> PKQLRFEGERVTWIQASTLKELLDLKAQHPEAKLVVGNTEIGIEMKFKNQLFPMIICPAWIPELNAVEHGPEGISFGAACALSSVEKTLLEAVAKLPTQKTEVFRGVLEQLRWFAGKQVKSVASLGGNIITASPISDLNPVFMASGTKLTIV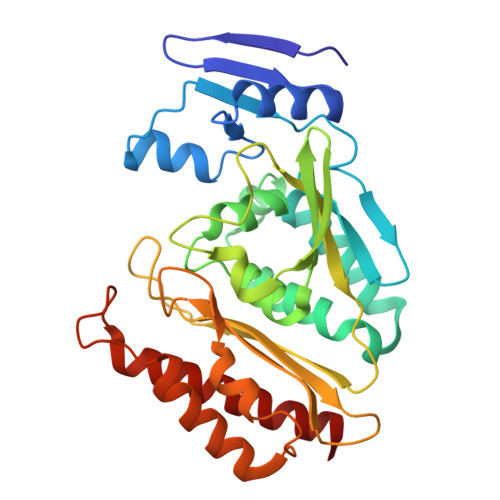SRGTRRTVPMDHTFFPSYRKTLLGPEEILLSIEIPYSREDEFFSAFKQASRREDDIAKVTCGMRVLFQPGSMQVKELALCYGGMADRTISALKTTQKQLSKFWNEKLLQDVCAGLAEELSLSPDAPGGMIEFRRTLTLSFFFKFYLTVLKKLG>[3x]GGGGGGMKPQLLALKQFVQTEFEKVDFETFRQNFNRCLEREQSTLLIYEDDDYDDQSFFLKPMLSDAFFI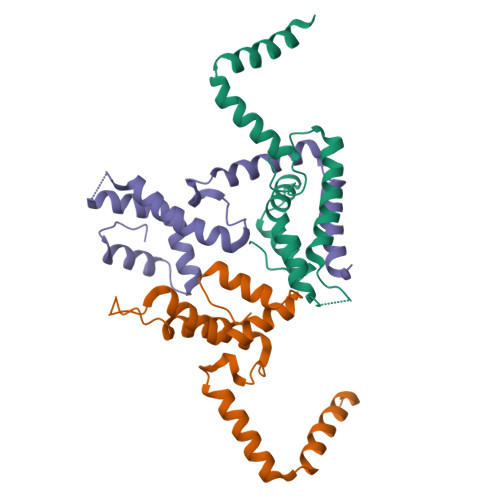SSEVVKQLDLLAVLVDNPKGDVKSCCQSFYEALTLFISALAITKGVDVGRYHQQLGKRFGVLTVY> SSLDDKPQFPGASAEFIDKLEFIQPNVISGIPIYRVMDR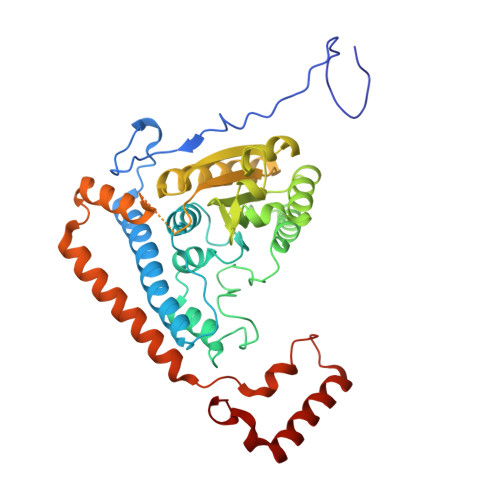QGQIINPSEDPHLPKEKVLKLYKSMTLLNTMDRILYESQRQGRISFYMTNYGEEGTHVGSAAALDNTDLVFGQFREAGVLMYRDYPLELFMAQCYGNISDLGKGRQMPVHYGCKERHFVTISSPLATQIPQAVGAAYAAKRANANRVVICYFGEGAASEGDAHAGFNFAATLECPIIFFCRNNGYAISTPTSEQYRGDGIAARGPGYGIMSIRVDGNDVFAVYNATKEARRRAVAENQPFLIEAMTYRIGHASTSDDSSAFRSVDEVNYWDKQDHPISRLRHYLLSQGWWDEEQEKAWRKQSRRKVMEAFEQAERKPKPNPNLLFSDVYQEMPAQLRKQQESLARHLQTYGEHYPLDHFDK> MNHKVHHHHHHIEGRHMPLNNYLHVFYYSWYGNPQFDGKYIHWNHPVLEHWDPRIAKNYPQGRHNPPDDIGSSFYPELGSYSSRDPSVIETHMRQMRSASIGVLALSWYPPDVNDENGEPTDNLVPTILDKAHKYNLKVTFHIEPYSNRDDQNMYKNVKYII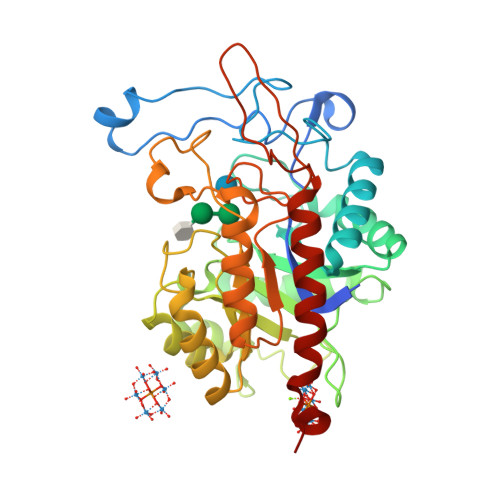DKYGNHPAFYRYKTKTGNALPMFYVYDSYITKPEKWANLLTTSGSRSIRNSPYDGLFIALLVEEKHKYDILQSGFDGIYTYFATNGFTYGSSHQNWASLKLFCDKYNLIFIPSVGPGYIDTSIRPWNTQNTRNRINGKYYEIGLSAALQTRPSLISITSFNQWHEGTQIEKAVPKRTSNTVYLDYRPHKPGLYLELTRKWSEKYSKERATYALDRQLPVS Cas12f, also known as Cas14, is an exceptionally small type V-F CRISPR–Cas nuclease that is roughly half the size of comparable nucleases of this type. Cas12f associates with a crRNA and a tracrRNA, which can be fused into a single guide RNA (sgRNA), to target substrate DNA. An asymmetric Cas12f dimer is bound to one sgRNA for recognition and cleavage of dsDNA substrate with a T-rich PAM sequence. Despite its small size, Cas12f contains all the conventional domains of Cas12 proteins, compared with other known Cas12 nuclease structures.

To understand the mechanism of Cas12f activation by target DNA, we determined the cryo-EM structure of Cas12f-sgRNA binary complex at 3.9 Å. This structure reveals a 5-nt pre-ordered seed sequence in the crRNA adjacent to the PAM duplex. The 5′ end seed sequence was also observed in other Cas12 nucleases, including Cas12a, Cas12b and Cas12i. The binary complex structure also allows us to reveal the conformational changes in Cas12f upon target DNA recognition. The most significant conformational changes happen in the C-terminal half of Cas12f.1 (RuvC, REC2 and Nuc) and N-terminal half of Cas12f.2 (REC1 and WED); both move outward upon the formation of the crRNA-target DNA heteroduplex between them. The lid motif of Cas12f.1 transits from the closed to open conformation, exposing the active site to accommodate ssDNA substrate. However, almost no conformational changes are observed in the RuvC domain of Cas12f.2, further suggesting that Cas12f.2 is not responsible for substrate cleavage. The conformational changes, particularly in the lid motif of Cas12f.1, are similar to those observed in Cas12a, Cas12b and Cas12i. Although both copies of the Cas12f effector protein are necessary for the complex's functionality, this evidence suggests that Cas12f still adopts a conserved mechanism for activation of the RuvC nuclease site like other type V nucleases.

>[2x]MAKNTITKTLKLRIVRPYNSAEVEKIVADEKNNREKIALEKNKDKVKEACSKHLKVAAYCTTQVERNACLFCKARKLDDKFYQKLRGQFPDAVFWQEISEIFRQLQKQAAEIYNQSLIELYYEIFIKGKGIANASSVEHYLSDVCYTRAAELFKNAAIASGLRSKIKSNFRLKELKNMKSGLPTTKSDNFPIPLVKQKGGQYTGFEISNHNSDFIIKIPFGRWQVKKEIDKYRPWEKFDFEQVQKSPKPISLLLSTQRRKRNKGWSKDEGTEAEIKKVMNGDYQTSYIEVKRGSKICEKSAWMLNLSIDVPKIDKGVDPSIIGGIDVGVKSPLVCAINNAFSRYSISDNDLFHFNKKMFARRRILLKKNRHKRAGHGAKNKLKPITILTEKSERFRKKLIERWACEIADFFIKNKVGTVQMENLESMKRKEDSYFNIRLRGFWPYAEMQNKIEFKLKQYGIEIRKVAPNNTSKTCSKCGHLNNYFNFEYRKKNKFPHFKCEKCNFKENADYNAALNISNPKLKSTKEEP> MKIRSQVGMVLNLDKCIGCHTCSVTCKNVWTSREGVEYAWFNNVETKPGQGFPTDWENQEKYKGGWIRK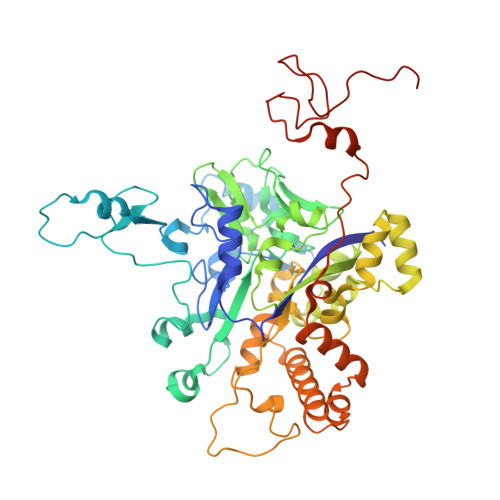INGKLQPRMGNRAMLLGKIFANPHLPGIDDYYEPFDFDYQNLHTAPEGSKSQPIARPRSLITGERMAKIEKGPNWEDDLGGEFDKLAKDKNFDNIQKAMYSQFENTFMMYLPRLCEHCLNPACVATCPSGAIYKREEDGIVLIDQDKCRGWRMCITGCPYKKIYFNWKSGKSEKCIFCYPRIEAGQPTVCSETCVGRIRYLGVLLYDADAIERAASTENEKDLYQRQLDVFLDPNDPKVIEQAIKDGIPLSVIEAAQQSPVYKMAMEWKLALPLHPEYRTLPMVWYVPPLSPIQSAADAGELGSNGILPDVESLRIPVQYLANLLTAGDTKPVLRALKRMLAMRHYKRAETVDGKVDTRALEEVGLTEAQAQEMYRYLAIANYEDRFVVPSSHRELAREAFPEKNGCGFTFGDGCHGSDTKFNLFNSRRIDAIDVTSKTEPHP2-methoxy-6-methyl-4-(4-methyl-3,4-dihydro-2H-1,4-benzoxazin-7-yl)phenol | C17 H19 N O3 | 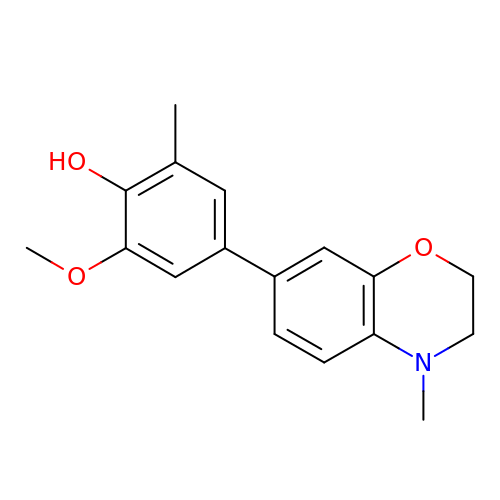RZARGVUVKRIAGU-UHFFFAOYSA-N> MKVGQDKVVTIRYTLQVEGEVLDQGELSYLHG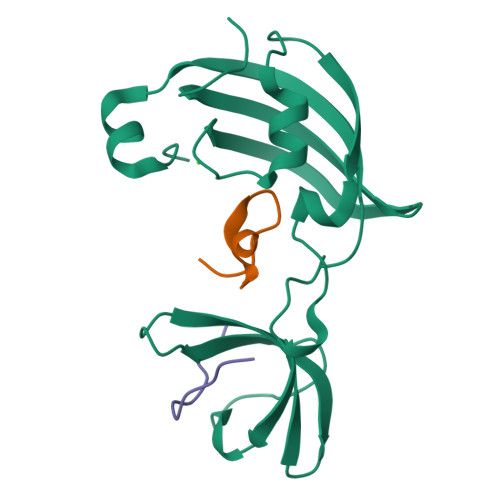HRNLIPGLEEALEGREEGEAFQAHVPAEKAYGPHDPEGVQVVPLSAFPEDAEVVPGAQFYAQDMEGNPMPLTVVAVEGEEVTVDFNHPLAGKDLDFQVEVVKVREATPEELLHGHAHPSGHHHHHH;>[2x]TRYANAKMLPFAFGA> SNATYQYNMNFEKLGKCIIINNKNFDKVTGMGVRNGTDKDAEALFKCFRSLGFDVIVYNDCSCAKMQDLLKKASEEDHTNAACFACILLSHGEENVIYGKDGVTPIKDLTAHFRGDRCKTLLEKPKLFFIQACRGTELDDGI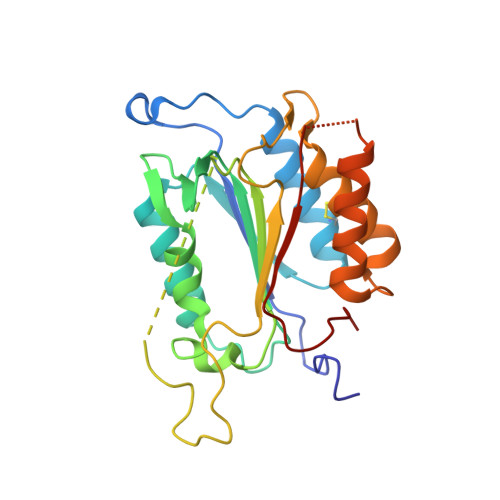QAASGPINDTDANPRYKIPVEADFLFAYSTVPGYYSWRSPGRGSWFVQALCSILEEHGKDLEIMQILTRVNDRVARHFESQSDDPHFHEKKQIPCVVSMLTKELYFSQ[[[(2~{R},3~{S},4~{R},5~{R})-5-(6-aminopurin-9-yl)-3,4-bis(oxidanyl)oxolan-2-yl]methoxy-oxidanyl-phosphoryl]oxy-sulfanyl-phosphoryl] [(2~{R},3~{R},4~{R},5~{R})-5-(2-azanyl-7-methyl-6-oxidanyl-purin-7-ium-9-yl)-4-methoxy-3-oxidanyl-oxolan-2-yl]methyl 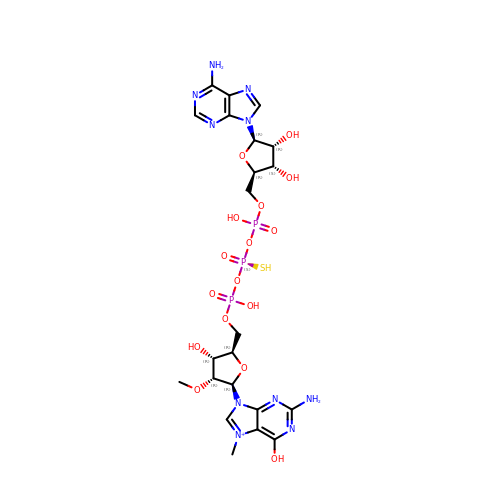hydrogen phosphate | C22 H32 N10 O16 P3 S | LVAVASOWNAXXPY-KVLYALRXSA-O>MAKWRCKICGYIYDEDEGDPDNGISPGTKFEDLPDDWVCPLC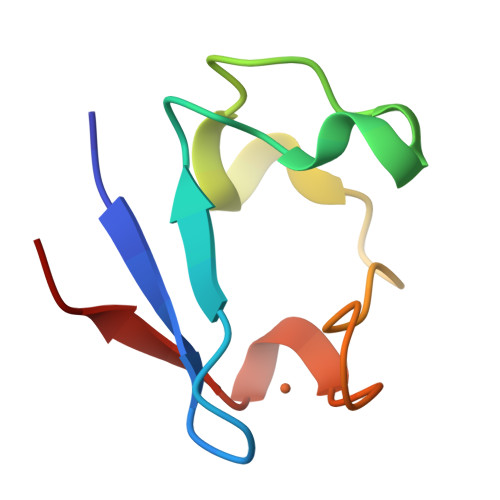GAPKSEFERIE[4x]>[5x]SRGTAGAPMRGYKVTDNERTRKYGIGA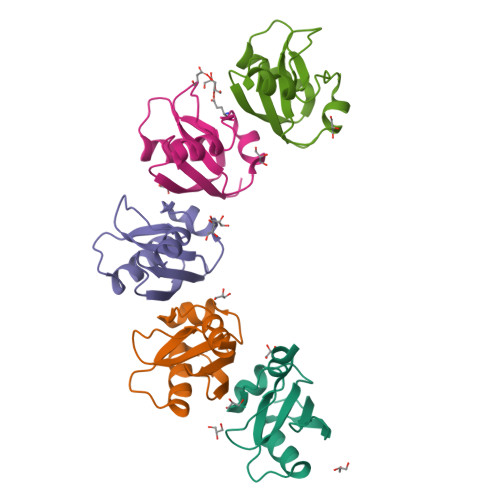NSLEMLIAKAKSKFPLLEPHLYLASDGFEVSDDEYLKSLPAQTLFIVSGPDAVITTDADFEFEKMLEHHHHHH> MENSISGLTEEQA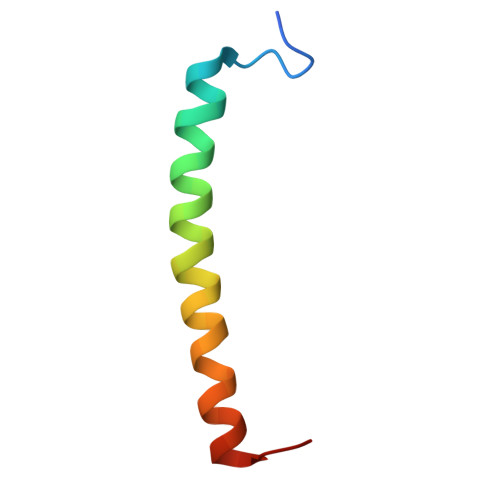KEFHEQFKVVFTTFVVLAAAAHFLVFLWRPWF>[10x]MLVFIDDGSTNIKLQWQESDGTIKQHISPNSFKREWAVSFGDKKVFNYTLNGEQYSFDPISPDAVVTTNIAWQYSDVNVVAVHHALLTSGLPVSEVDIVCTLPLTEYYDRNNQPNTENIERKKANFR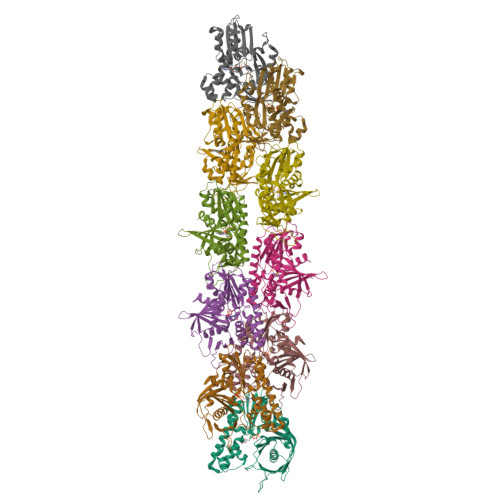KKITLNGGDTFTIKDVKVMPESIPAGYEVLQELDELDSLLIIDLGGTTLDISQVMGKLSGISKIYGDSSLGVSLVTSAVKDALSLARTKGSSYLADDIIIHRKDNNYLKQRINDENKISIVTEAMNEALRKLEQRVLNTLNEFSGYTHVMVIGGGAELICDAVKKHTQIRDERFFKTNNSQYDLVNGMYLIGN>MTSIYPKFRAAAVQAAPIYLNLEASVEKSCELIDEAASNGAKLVAFPEAFLPGYPWFAFIGHPEYTRKFYHELYKNAVEIPSLAIRKISEAAKRNETYVCISCSEKDGGSLYLAQLWFNPNGDLIGKHRKMRASVAERLIWGDGSGSMMPVFQTEIGNLGGLMCWEHQVPLDLMAMNAQNEQVHVASWPGYFDDEISSRYYAIATQTFVLMTSSIYTEEMKEMICLTQEQRDYFETFKSGHTCIYGPDGEPISDMVPAETEGIAYAEIDVERVIDYKYYIDPAGHYSNQSLSMNFNQQPTPV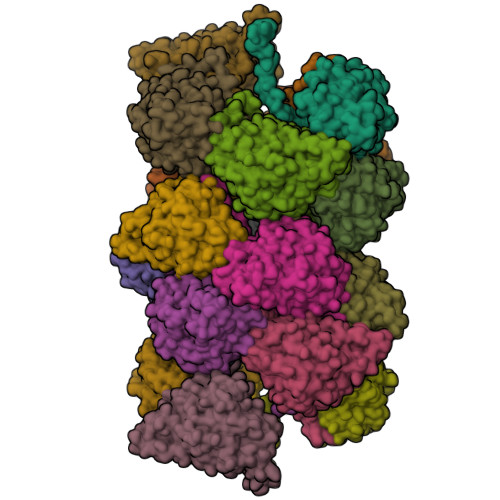VKKLNKQKNEVFTYEDIQYQKGILEEKV[18x]>GGDSRELIARYQILLAELAAIRADIAAERTGDPYVRKLARELKRLAQEAAEEVKRDPSSSDVNMALLLILLMIELAVRALEAAERTGDPEVRELAAELVWLAVEAAEEVQRNPSSSDVWLALHLIMLAIWAAVAALEAAERTGDPEVRELARELVRLAVEAAEEVQRNPSSKEVY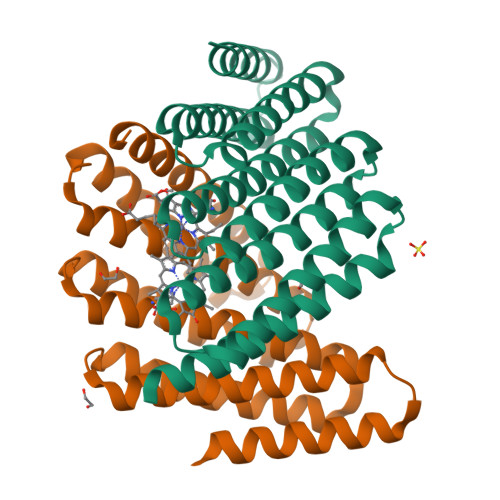MALLLILIAILEAVLSLLRAERSGDPEKREKARERVREAVERAEEVQR[2x]> AVIPILVIACDRSTVRRCLDKLLHYRPSAELFPIIVSQDCGHEETAQVIASYGSAVTHIRQPDLSNIAVQPDHRKFQGYYKIARHYRWALGQIFHNFNYPAAVVVEDDLEVAPDFFEYFQATYPLLKADPSLWCVSAWNDNGKEQMVDSSKPELLYRTDFFPGLGWLLLAELWAELEPKWPKAFWDDW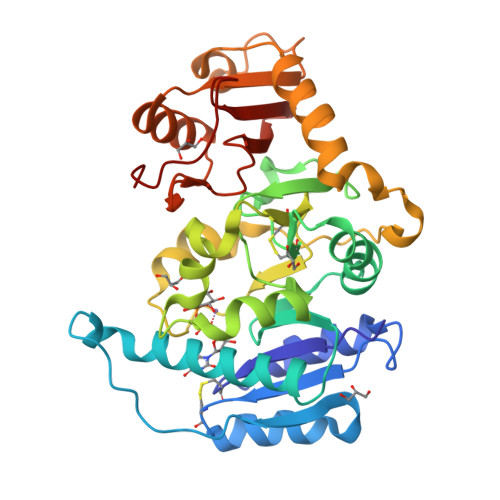MRRPEQRKGRACVRPEISRTMTFGRKGVSHGQFFDQHLKFIKLNQQFVPFTQLDLSYLQQEAYDRDFLARVYGAPQLQVEKVRTNDRKELGEVRVQYTGRDSFKAFAKALGVMDDLKSGVPRAGYRGIVTFLFRGRRVHLAPPQTWDGYDPSWT>[2x]GSFTEELHLIPP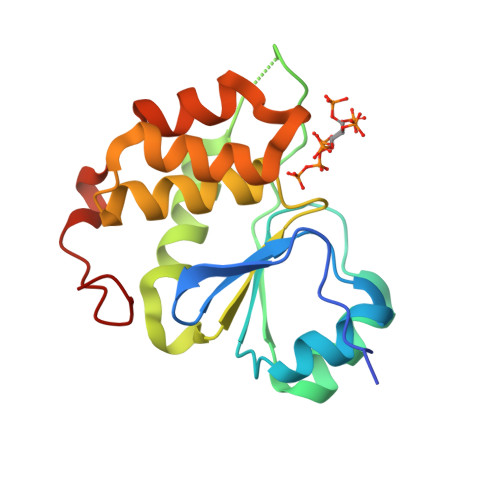LNFSMVDNGIFRSGFPDSANFSFLQTLGLRSIIYLCPEPYPESNLQFLKSNGIRLFQFGIEGNKEPFVNIPDHKIRMALKVLLDEKNHPVLIHSKRGKHRTGCLVGCLRKLQKWCLTSIFDEYQRFAAAKARVSDQRFMEIFDVSSFSHIPMSFSCSIR>[2x]MDPLCAAPCSCDGDRRVDCSGKGLTAVPEGLSAFTQALDISMNNITQLPEGAFKNFPFLEELQLAGNDLSFIHPKALSGLKELKVLTLQNNQLKTVPSEAIRGLSALQSLRLDANHITSVPEDSFEGLVQLRH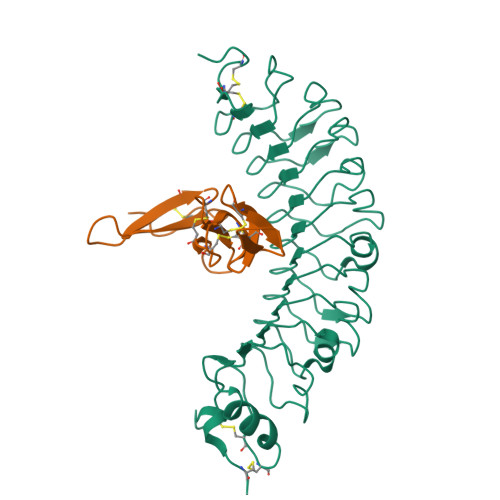LWLDDNSLTEVPVHPLSNLPTLQALTLALNKISSIPDFAFTNLSSLVVLHLHNNKIRSLSQHCFDGLDNLETLDLNYNNLGEFPQAIKALPSLKELALDTNQLKSVPDGIFDRLTSLQKIWLHTNPWDCSCPRIDYLSRWLNKNSQKEQGSAKCSGSGKPVRSIICPT;>[2x]AEGSQACAKGCELCSEVNGCLKCSPKLFILLERNDIRQVGVCLPSCPPGYFDARNPDMNKCIKCKIEHCEACFSHNFCTKCKEGLYLHKGRCYPACPEGSSA> XSFALGLRKDCRAEIVEKFTEPGTVI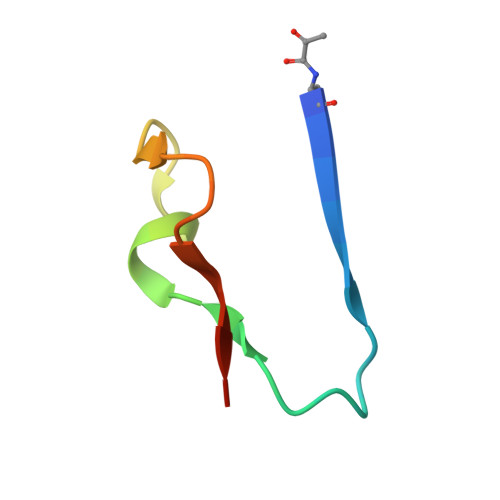RINEVVAALKA>[8x]MSYTVGTYLAERLVQIGLKHHFAVAGDYNLVLLDNLLLNKNMEQVYCCNELNCGFSAEGYARAKGAA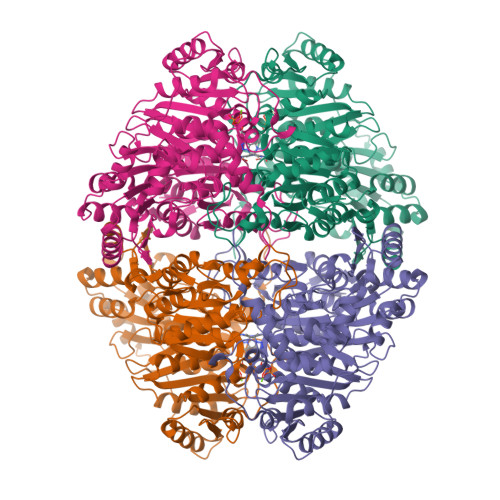AAVVTYSVGALSAFDAIGGAYAENLPVILISGAPNNNDHAAGHVLHHALGKTDYHYQLEMAKNITAAAEAIYTPEEAPAKIDHVIKTALREKKPVYLEIACNIASMPCAAPGPASALFNDEASDEASLNAAVEETLKFIANRDKVAVLVGSKLRAAGAEEAAVKFADALGGAVATMAAAKSFFPEENPHYIGTSWGEVSYPGVEKTMKEADAVIALAPVFNDYSTTGWTDIPDPKKLVLAEPRSVVVNGIRFPSVHLKDYLTRLAQKVSKKTGALDFFKSLNAGELKKAAPADPSAPLVNAEIARQVEALLTPNTTVIAETGDSWFNAQRMKLPNGARVEYEMQWGHIGWSVPAAFGYAVGAPERRNILMVGDGSFQLTAQEVAQMVRLKLPVIIFLINNYGYTIEVMIHDGPYNNIKNWDYAGLMEVFNGNGGYDSGAGKGLKAKTGGELAEAIKVALANTDGPTLIECFIGREDCTEELVKWGKRVAAANSRKPVNKLL> LDFSKWKTRQPGEFRAPCPAMNSLANHGFIPRDGRNITVAMLVPVLQEVFHLSPELAQTISTLGLFTAQDPSKGVFTLDDLNRHNLFEHDASLSREDYYFHKDASTFRPEVFKKFMSHFKGKEYVTLEDAASARYAMVQESRKKNPTFTYTVQQRITSYGETIKYFRTIVEPATGKCPVAWIKILFEQERLPYNEGWRPPKAELSGFSMASDVLELALVTPEKLID;> ALDFSKWKTRQPGEFRAPCPAMNSLANHGFIPRDGRNITVAMLVPVLQEVFHLSPELAQTISTLGLFTAQDPSKGVFTLDDLNRHNLFEHDASLSREDYYFHKDASTFRPEVFKKFMSHFKGKEYVTLEDAASARYAMVQESRKKNPTFTYTVQQRITSYGETIKYFRTIVEPATGKCPVAWIKILFEQERLPYNEGWRPPKAELSGFSMASDVLELALVTPEKLID

Unspecific peroxygenases (UPOs) are enzymes catalyzing the oxyfunctionalization of both aromatic and aliphatic molecules, including specific products that are difficult to be obtained only by chemical means. Therefore, they are of high biotechnological interest for the regio- and/or stereoselective synthesis of biobased compounds and other fine chemicals and pharmaceuticals. These enzymes form a group of fungal heme-thiolate peroxidases (HTPs). Hence, they share a proximal cysteine residue acting as the fifth ligand of the heme iron with the phylogenetically distant cytochrome P450 monooxygenases (P450s), present in all living organisms. In the present study, two UPOs from the basidiomycete Marasmius rotula (rMroUPO) and the ascomycete Collariella virescens (rCviUPO) were crystallized after sequence optimization and Escherichia coli expression as active soluble enzymes.

The rCviUPO asymmetric unit reveals a compact dimer through a parallel association of helix α12 from each monomer, providing a closely packed helix interface. The rCviUPO structure includes all amino acid residues, except for the initial Glu1 and the thirty-two C-terminal residues—from Lys228 to Lys259, whose lack is due to their flexible conformation—one heme molecule and one Mg2+ ion. The monomer adopts an α fold formed by twelve helices and two short β strands (E124-V126 and K177-P179). In rCviUPO, the neighbor residues located at the upper side of the cofactor that outline the cavity shell include Leu57, Ile61, His90, Phe88, Gly161, Glu162, and Lys165, with the heme iron coordinated by the thiol side chain of Cys19 at the lower side. The Mg2+-coordinating residues in rCviUPO (at 2.01–2.14 Å) are the same found in rMroUPO, but no acetate was found at the heme pocket. This is in agreement with its absence from the rCviUPO crystallization medium, and resulted in the presence of one water molecule (wat255) near the sixth coordination position of the heme iron. Phe160 of rMroUPO was replaced by Lys165 in rCviUPO and, as a result of this and other amino acid substitutions, the access to the substrate binding site in rCviUPO was narrowed. In the rCviUPO crystal structure, the buried interface area of the dimer, including the two α12 helices, was 1304 Å2. Dominant at the upper side of the interface are Arg156 and Lys224, which establish polar contacts on both sides with residues Glu216 and Glu223, respectively. At the corner of the dimer, Ser54 and Glu56 also bridge the interface by hydrogen bond interactions.> MRTDKEIFVSVDVETSGPIPGKYSMLSIGACVAFEPSKQFSCYLKPISEDFIPAAMEVTGLSLEKLHVDGLDPVDAMVQFKEWINSVVKEDETVVFVGFNASFDWSFINYYFHVYLGDNPFGIAALDIKSMYFGVSHASWRLTRSSEIAKVVKPETYGDHDALHDARYQAELFRL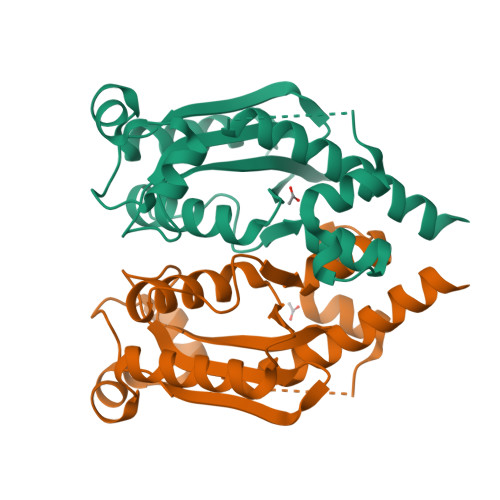IDKLSEKKKLDR> MNDLERLFNPSAIAVVGASKDPSKIGSQILRNLLSYGFKGKVYPINPTADELMGLKCYPKVSDVPDKVDVAVISVPSDKVLGVIDDCGKAGVKFAVVITSGFKEVGNEELEEELVRRAHSYGMRVLGPNIFGYLYAPARLNATFGPKDVLSGNVAFISQSGALGIALMGYTVVENIGISS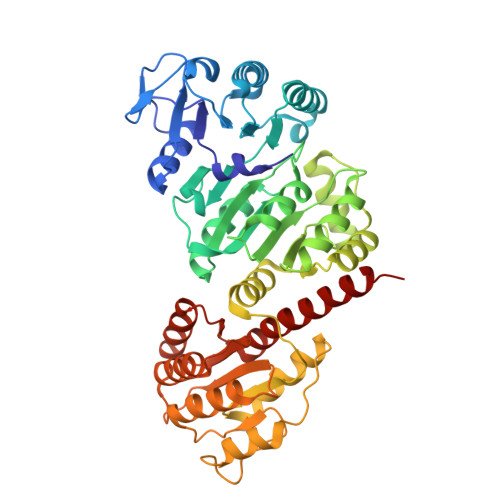IVSVGNKADLDDVDLLDFFDKDPNTGVIMIYLEGIAPGRGRMFIDVASRVSLRKPIIVIKAGRTEVGARAAASHTGSIAGSVAIYESAFKQSGILMAKSVEDAFDWTKALSWNPIPEGERLIVLTNGGGAGVQSTDTFADNGIYLSKPPESLIQEIKKFVPPFASFANPIDITGMAPDDWYYMGTLAALKNPDVDALTVLYCQTAVTTPIGVAKGIVDAIKEAGNSKPVTVGMVGGPEVAEAVSFLNKQRIAAYPTPERASSAMSALYAYARARSYVMKSLAVR>GDGTKVEELNKATAAMMVPFDSVKFTGNYGNMTEISYQVAKRAAKKGAKYYHITRQWQERGNNITISADLYK[2x]

The DUF1471 family includes several hundred members, all occurring exclusively in the Enterobacteriaceae, such as Escherichia, Salmonella, Yersinia, and Shigella, among others. Many of the basic features of sequences in the family of conserved proteins from Enterobacteriaceae now known as DUF1471 (PF07338, alternatively, the YhcN or BhsA/McbA family) were recognized soon after release of the first E. coli genome sequence. These proteins are characteristically small, single domain proteins of around 90 residues; though one subfamily has three repeated DUF1471 domains. Most DUF1471 sequences contain apparent signal sequences that target them to the periplasm. The fold features a three-stranded antiparallel β-sheet with another, shorter N-terminal β-strand parallel to strand 3, so that the strands are ordered 2-4-3-1 across the sheet, with strands 1 and 3 parallel.

SssB (STM1478, also known as YdgH) is another Salmonella DUF1471 paralogue implicated in pathogenesis. SssB and its homologues contain three DUF1471 domains (I, II, and III). The structure of the C-terminal domain (III) of SssB was determined by X-ray crystallography by the Midwest Center for Structural Genomics (MCSG); target ID APC101565. Protein crystals diffracting to resolution suitable for structure determination were only obtained in case of the fragment 244–314 corresponding to the SssB-III DUF1471 domain, and for this reason the solution state structure of SssB-I was solved by NMR spectroscopy. Despite the fact that the crystals were pseudo-merohedrally twinned, the SssB-III structure was determined by single-wavelength anomalous diffraction. The final atomic model refined to 1.45 Å resolution and contained two molecules (A and B) in the asymmetric unit. The molecule A of SssB-III structure comprises residues Lys 247 to Glu 301 and Asn 305 to Lys 314 whereas molecule B comprises residues Lys 247 to Lys 314. The SssB C-terminal domain (SssB-III) adopts a dimeric form in the X-ray structure. However, the relative arrangement of monomers and the dimer interface are different from those of SrfN, and likely represent a crystallization artifact. In the SssB-III X-ray structure, residues in loop 2 and in the neighboring transition (loop 1) from strand 2 into the long helix exhibited particularly high B-factors and are likely to be locally flexible in solution.> MAEQPPETHRFVDDYLPALLAQASQLISSEFHEVARQHGFSVSEWRVMASLAGSEPISIGQLAQVTVTKQPTVTRLLDRMEARGQVERLPHESDRRITLVRITRKGLKAVEHLMELAREHERRVLEPFGLRRAEELKQTLRQMIDLHVHVPVEEPEED

We characterize the binding of IAA to MarR-family regulators from both iac and iad loci. Most characterized MarR-family regulators function as repressors by binding to an operator sequence upstream of the genes they control. When a relevant ligand binds the MarR repressor, it releases from DNA, allowing gene expression. The structures of MarRs from representatives of each auxin degradation operon type establish that each has distinct IAA-binding pockets.

We recombinantly produced the two MarR proteins from the auxin degradation locus of V. paradoxus CL14, MarR_73 (IadR) and MarR_50 (IadR2), and employed isothermal titration calorimetry to determine their binding affinities for IAA, other auxins and related aromatic compounds. Eleven additional auxin and aromatic ligands were examined, with ten exhibiting lower affinities for MarR_73 than that of IAA. MarR_73 structures complexed with nine other auxins were also determined and refined to 1.35–1.6 Å resolution. The MarR_73 structures resolved in complexes with other auxins revealed that the positions of ligand-contacting regions remained unchanged upon the binding of auxins, with the exceptions of the His-32 imidazole ring, which shifted by up to 2.9 Å, and the Arg-46 guanidinium group, which shifted by up to 4.2 Å. In both cases, these shifts accommodated differences in the carboxylate-containing substituent groups of the auxins examined.>[3x]MSKQFVRSAKNLVKGYSSTQVLVRNATSNDNHQVSKDSLIELAEKSYDSADFFEIMDMLDKRLNDKGKYWRHIAKALTVIDYLIRFGSENCVLWCRENLYIIKTLKEF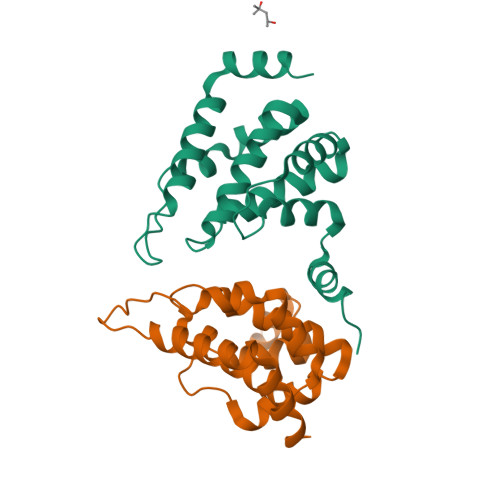RHEDDEGIDQGQIVRVKAKELTALLSDDERLNEERNMNIKGRNRKG>MNYARFITAASAARNPSPI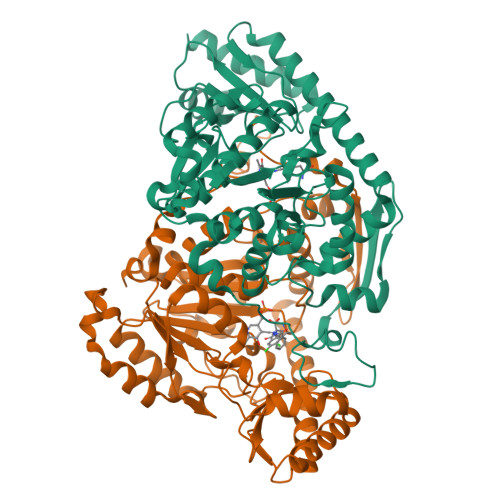RTMTDILSRGPKSMISLAGGLPNPNMFPFKTAVITVENGKTIQFGEEMMKRALQYSPSAGIPELLSWLKQLQIKLHNPPTIHYPPSQGQMDLCVTSGSQQGLCKVFEMIINPGDNVLLDEPAYSGTLQSLHPLGCNIINVASDESGIVPDSLRDILSRWKPEDAKNPQKNTPKFLYTVPNGNNPTGNSLTSERKKEIYELARKYDFLIIEDDPYYFLQFNKFRVPTFLSMDVDGRVIRADSFSKIISSGLRIGFLTGPKPLIERVILHIQVSTLHPSTFNQLMISQLLHEWGEEGFMAHVDRVIDFYSNQKDAILAAADKWLTGLAEWHVPAAGMFLWIKVKGINDVKELIEEKAVKMGVLMLPGNAFYVDSSAPSPYLRASFSSASPEQMDVAFQVLAQLIKESL[2x]4-[(E)-2-[1-(7-chloranylheptyl)pyridin-1-ium-4-yl]ethenyl]-N,N-dimethyl-aniline | C22 H30 Cl N2 | 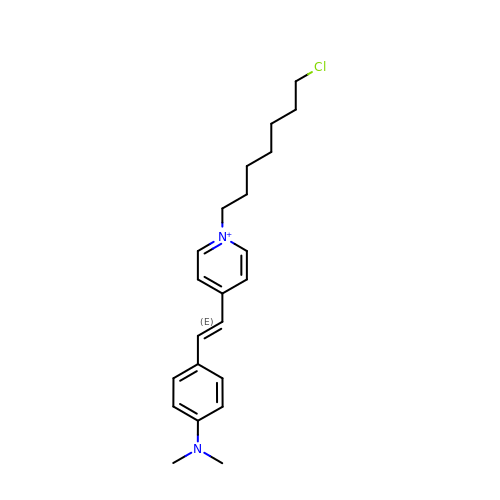WTHMXSWCQZGWBE-UHFFFAOYSA-N Most extensively studied in this group are the F-specific filamentous phages (Ffs) that include viruses f1, fd and M13. Ffs are also strikingly simple—their single-stranded DNA genome encodes just 11 proteins, of which 5 form the phage capsid. pVIII is the major capsid protein that forms the filamentous body of the phage. The tips of the filament are formed of the minor capsid proteins which occur in pairs. pIII and pVI form the leading end of the infecting phage, which interacts with the host receptors to initiate entry, whereas pVII and pIX form the trailing end11,12.

pVII and pIX are small hydrophobic proteins of only 33 and 32 amino acids, respectively. They both lack a signal sequence, form a single α-helix, and are present at the tip in 5 copies each. 5 copies of pVII form a helical bundle, packed together using mainly hydrophobic interactions. The terminus of the round end of the phage is comprised of the N-terminus of pVII, which is mostly negatively charged. In our map, density is missing for five residues as the far N-terminus of pVII, which would contribute to the negative charge and be of mixed hydrophobicity. In layer 1, 10 helices of alternating pIX and pVIII line the outside of the pVII bundle. Interactions are mainly hydrophobic, with salt bridges between pIX and pVII subunits, and hydrogen bonds between pIX and pVIII subunits, adding further stability to the tip structure. Further copies of the main capsid protein pVIII continue to coat the round tip in two further layers (layers 2–3), interacting with the pIX helices by mostly hydrophobic interactions. The helical symmetry of the filament is slightly altered as it comes close to the round tip, presumably because of the slightly altered binding partners, and the change from helical symmetry of the filament to only 5-fold symmetry at the very tip. At the round end, the 5 C-terminal arginine residues of pVII (Arg 33) and 5 arginine residues from pIX (Arg 26) form a positively charged ring that butts up to the tip of the DNA, where the packaging hairpin is expected to be found.

>[45x]AEGDDPAKAAFDSLQASATEMIGYAWAMVVVIVGATIGIKLFKKFTSKAS;>[5x]MEQVADFDTIYQAMIQISVVLCFALGIIAGGQR;>[5x]MSVLVYSFASFVLGWCLRSGITYFTRLMETSS> MGSSHHHHHHSSGLVPRGSEDYNFVFKVVLIGESGVGKTNLLSRFTRNEFSHDSRTTIGVEFSTRTVMLGTAAVKAQIWDTAGLERYRAITSAYYRGAVGALLVFDLTKHQTYAVVERWLKELYDHAEATIVVMLVGNKSDLSQAREVPTEEARMFAENNGLLFLETSALDSTNVELAFET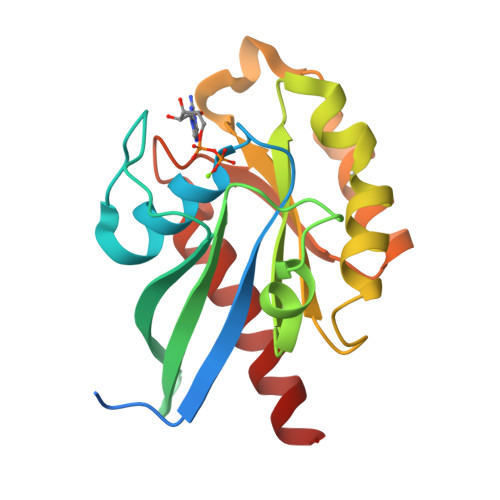VLKEIFAKVSKQ> GAQRPRGPQRGKDIKHEISASLEELYKGRTAKLALNKQILCKECEGRGGKKGAVKKCTSCNGQGIKFVTRQMGPMIQRFQTECDVCHGTGDIIDPKDRCKSCNGKKVENERKILEVHVEPGMKDGQRIVFKGEADQAPDVIPGDVVFIVSERPHKSFKRDGDDLVYEAEIDLLTAIA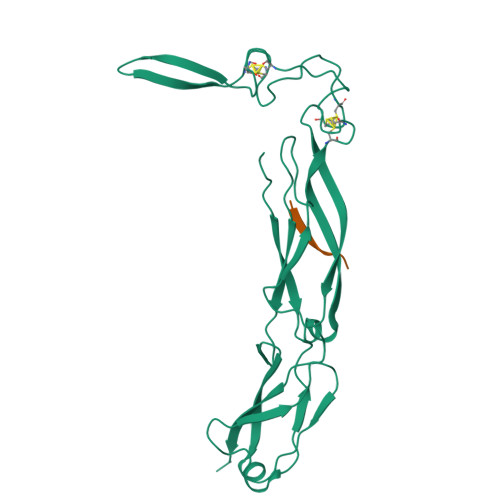GGEFALEHVSGDWLKVGIVPGEVIAPGMRKVIEGKGMPIPKYGGYGNLIIKFTIKDPENHFTSEENLKKLE;> GWLYEIS> ALRIDYPAALQILMEGGTHMVCTGRTHTDRICRFKWLCYSNEAEEFIFFHGNTSVMLPNLGSRRFQPALLDLSTVEDHATQYFNFVELPAAALRFMPKPVFVPDVALIANRFNPDNLMHVFHDDLLPLFYTLRQFPGLAHEARLFFMEGWGEGAHFDLYKLLSPKQPLLRAQLKTLGRLLCFSHAFVGLSKITTWYQYGFVQPQGPKANILVSGNEIRQFARFMTEKLNVSATGVPLGEEYILVFSRTQNRLILNEAELLLALAQEFQMKTVTVSLEDHTFADVVRLVSNASMLVSMHGAQLVTTLFLPRGATVVELFPYAVNPDHYTPYKTLAMLPGMDLQYVAWRNMMPENTVTHPERPWDQGGITHLDRAEQARILASREVPRHLCCRNPEWLFRIYQDTKVDIPSLIQTIRRVVKGRPGPRKQKWAAGLYPGKVREARCQASVHGASEARLTVSWQIPWNLKYLKVAEVKYEVWLQEAGEAAYVPYILALQNHTFTENIKP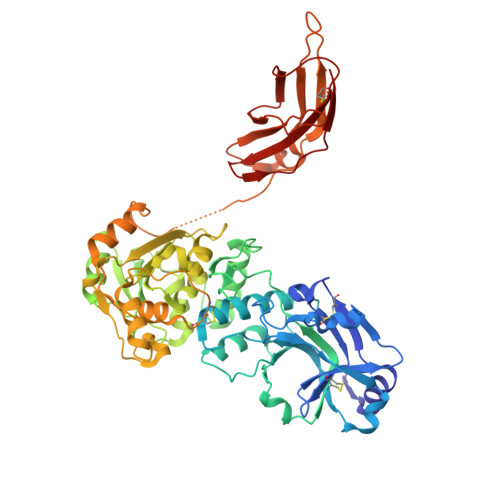FTTYLVWVRCIFNKILLGPFADVLVCNT>[2x]SMELATMGKVNEVLFMNGGEGEISYAQNSSFTEKVASMAMPALENAVETLFSKDFHLLPALNAADLGCAAGPNTFAVISMIKRMMEKKCRELYCQTPELQVYLNDLFGNDFNTLFKGLSSEVVGNKCEEVSCYVMGVPGSFHGRLFPRNSLHLVHSSYSVHWLTQAPKGLTSREGLALNKGKIYISKTSPPAVKEAYLSQFHEDFTMFLNARSQEVVPNGCMVLILHGRQSSDPSEMESCFTWELLAIAIAELVSQGLIDEDKLDTFNVPSYFPSLEEVKDIVERDGSFTIDHLEGFELDSLEMQENDKWVRGDKFAKMVRAFTEPIISNQFGHEIMDKLYDKFTHIVVSDLEAELPKTTSIILVLSKIVG

Here, we identified three N-methyltransferases involved in the biosynthesis of caffeine from the leaves of Kucha. Combined with enzymatic study and kinetic analysis, we found that one of the N-methyltransferases, CkTcS, serves as the critical N9-methyltransferase, which only acts on 1,3,7-trimethyluric acid but not caffeine, indicating that C8-oxidation must take place prior to N9-methylation. The structural characterization of CkTcS identified key residues around the substrate binding pocket that are critical for N9-methyltransferse activity. A previous study using 14C labeled caffeine has confirmed that theacrine is biosynthesized from caffeine, possibly initiated by oxidation at C8 to yield the intermediate 1,3,7-trimethyluric acid followed by N9-methylation.

We next asked why CkTcS prefers 5, given the fact that it shares a sequence identity >90% with CkTbS and CkCS. We tried to solve the structure of CkTbS and CkCS in the presence of SAH and their corresponding substrates, but only crystallized CkTbS. Unfortunately, the N-terminal cap domain of CkTbS is disordered due to crystal packing. We finally solved the structure of CkTbS in apo form. However, when overlapping the CkTbS and CkTcS structures, most residues lining the substrate binding pockets are in the same orientation, suggesting that substrate binding does not induce large conformational changes in the methyltransferase domain. The substrate specificity of CkTcS proteins might be determined by minor variable residues which subtly tailor the chemical features of the core catalytic scaffold. Further observation identified three sequence-variable residues around the pocket: CkTcS_Arg-226 (CkTbS_His-226, CkCS_Arg-225), CkTcS_Ile-241 (CkTbS_Thr-241, CkCS_Thr-240), and CkTcS_Cys-270 (CkTbS_Ser-270, CkCS_Ser-269). In CkTbS and CkCS, Ile-241 is replaced by a threonine, and Cys-270 by a serine, both of which contain hydrophilic side-chains that may introduce extra direct or water-mediated hydrogen-bond and influence substrate binding. Consistently, CkTbS H226R mutation led to an apparent increase of N9-methylation activity towards 5. Single mutation of T241I or C270S on CkTbS led to a moderate increase in reaction products, while the double and triple mutations further increased the N-methyltransferase activity to almost half of that of CkTcS.> GSHMEAVQNRIVEAAERVPGVRGVIHLRARYVGQDIWAHMIIGVDPENTVEQAHEICEAVQAAV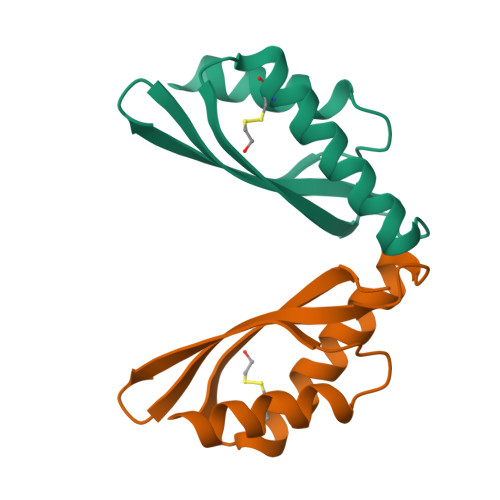CGKIRRIESLDVSAEAREIGDTTKPSFSDQPLSFDEVMLSKVDN To improve the understanding of molecular interactions between xenon and transmembrane receptor targets, we investigated xenon binding with the Gloebacter violaceus ligand-gated ion channel (GLIC), a member of the pLGIC family, using X-ray crystallography under pressurized gas. Previously, the sensitivity of GLIC to gaseous anesthetics has been studied using 2-electrode voltage clamping techniques and this revealed that GLIC currents are inhibited by clinical concentrations of xenon. GLIC, whose X-ray structures has been solved in open, locally-closed (LC)–inactive- and resting-state conformations, is extensively used to identify binding sites of general anesthetics, channel blockers, alcohols, and other allosteric modulators in pLGICs. Here, we show by X-ray diffraction that xenon has multiple and specific binding sites in GLIC either in the open and LC (inactive) conformations, and that these binding sites differ between the two conformations.

In the GLIC LC form, the bottom end of the cavity is obstructed because of a revolving motion of helix M2 and the M2-3 loop, and a conformational flip of the Y197 side chain. Upon channel closure, the revolving motion of the M2-3 loop destabilises this network of interactions and Y197 predominantly adopts a downward conformation stabilized through hydrogen bonding with T255 (M3 helix). Indeed, the xenon-bound GLIC LC structure reveals that the contraction of the intra-subunit cavity constrains xenon binding to one single location at the cavity entrance. This unique xenon binding site has a markedly lower occupation (0.7) than the xenon intra-subunit sites in GLIC open form (0.9–1.0) further illustrating that the reshaping of the intra-subunit cavity in GLIC LC form limits xenon-binding to this cavity. Xenon binds to a novel site located in the pore, in (and only in) GLIC LC form. This site is located in the middle of the channel pore, on the receptor five-fold symmetry axis, between the S230 and I233 rings of residues (respectively S6’ and I9’ in a prime notation that starts from the N-terminus of M2 helix). The inward movement of the M2 helices that occurs during the pore closure reduces the pore radius at position I233 (I9’) from 6 Å in GLIC open to 4 Å in GLIC LC and likely enables optimal hydrophobic interactions with xenon. The Xe atom is surrounded by the side chains of five Ile 233 (I9’) residues at a distance of 4.4 Å. In GLIC open form, xenon binds between M1 and M2 helices from one subunit and M2 helix from the adjacent subunit in the inner part of the TMD while in GLIC LC form, xenon binds between M1 helix from one subunit and M2 and M3 helices from the adjacent subunit in the outer part of the TMD. The location of a xenon atom in a functionally critical region of the pore could easily account for the inhibitory effect of xenon on GLIC.

>[5x]AQDMVSPPPPIADEPLTVNTGIYLIESYSLDDCAETFKVNAFLSLSWKDRRLAFDPVRSGVRVKTYEPEAIWIPEIRFVNVENARDADVVDISVSPDGTVQYLERFSARVLSPLDFRRYPFDSQTLHIYLIVRSVDTRNIVLAVDLEKVGKNDDVFLTGWDIESFTAVVKPANFALEDRLESKLDYQLRISRQYFSYIPNIILPMLFILFISWTAFWSTSYEANVTLVVSTLIAHIAFNILVETNCPKTPYMTYTGAIIFMIYLFYFVAVIEVTVQHYLKVESQPARAASITRASRIAFPVVFLLANIILAFLFFGF>MGKKFIVVCGNITVDSVTAFLRNFLRDKSGEINTEIVFLGETPPSLELETIFKCYLAYTTFISGSAMKWEDLRRVAVESAEACLIIANPLCSDSHAEDISNIMRVLSIKNYDSTTRIIIQILQSHNKVYLPKIPSWNWDTGDNIICFAELKLGFIAQGCLVPGLCTFLTSLFVEQNKKVMPKQTWKKHFLNSMKNKILTQRLSDDFA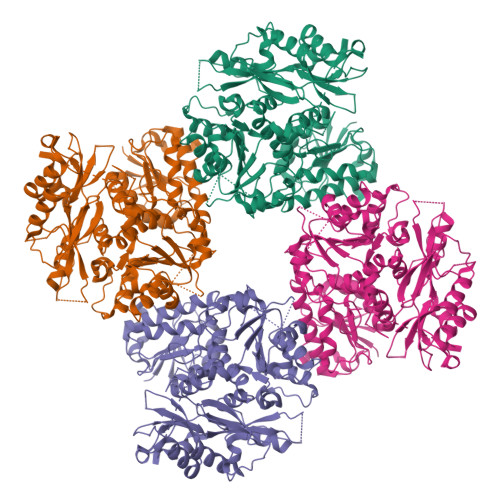GMSFPEVARLCFLKMHLLLIAIEYKSLFTDGFCGLILNPPPQVRIRKNTLGFFIAETPKDVRRALFYCSVCHDDVFIPELITNCGCKSRSRQHITVPSVKRMKKCLKGISSRISGQDSPPRVSASTSSISNFTTRTLQHDVEQDSDQLDSSGMFHWCKPTSLDKVTLKRTGKSKYKFRNHIVACVFGDAHSAPMGLRNFVMPLRASNYTRKELKDIVFIGSLDYLQREWRFLWNFPQIYILPGCALYSGDLHAANIEQCSMCAVLSPPPQPSSNQTLVDTEAIMATLTIGSLQIDEKSNCRKVPILTELKNPSNIHFIEQLGGLEGSLQETNLHLSTAFSTGTVFSGSFLDSLLATAFYNYHVLELLQMLVTGGVSSQLEQHLDKDKVYGVADSCTSLLSGRNRCKLGLLSLHETILSDVNPRNTFGQLFCGSLDLFGILCVGLYRIIDEEELNPENKRFVITRPANEFKLLPSDLVFCAIPFSTACYKRNEEFSLQKSYEIVNKASNSLEVLFQ[2x]> GPLGSGDVQVTEDAVRRYLTRKPMTTKDLLKKFQTKKTGLSSEQTVN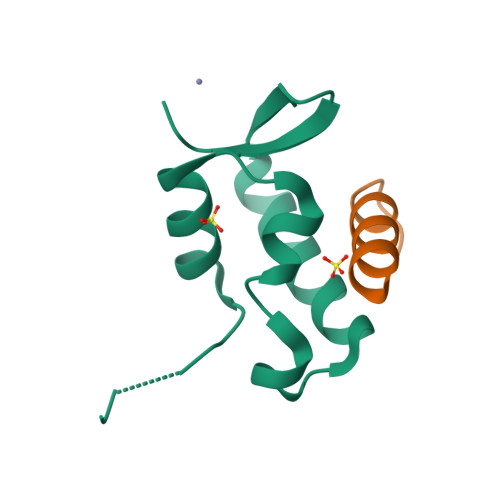VLAQILKRLNPERKMINDKMHFSLKE;> SEADEMAKALEAELNDLM2-(4-chlorophenyl)-4-[(3S)-piperidin-3-ylamino]thieno[2,3-d]pyridazine-7-carboxamide 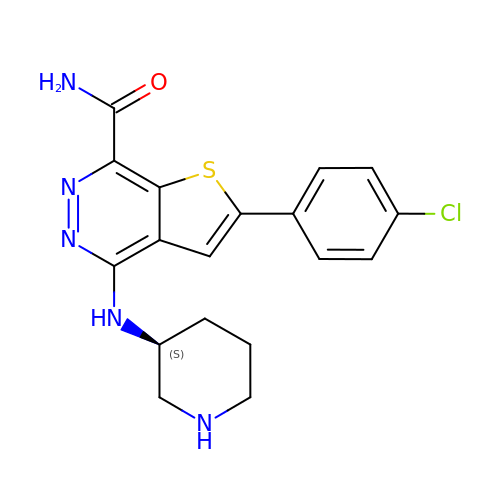| C18 H18 Cl N5 O S | OIVCIDIQAWPEAZ-LBPRGKRZSA-N> SQCSGIDKRDFIQGVSGGTWVDVVLDRKGCVTISATGKPTIDVRMVKMEASNLASVRTYCLEASTSEISSVNGCPSTTEAHNDKRKDSTYLCERSYPDRGWGNGCGLFGRGSLDTCVKFACSKKMAGHAISRENIVITAAVSVHGHSGAESDDRSQRKSRKELAELTITFKSSIVEADLGDYGKVQFECLMDFGIDLDDVYTADMSGKWWLVKRDWYHDIALPWTAPSADFWHDMDRLVEFSTPHATKQSVYTLGDQEGAMSTALGDAAVIEYMSSGSKVVFRTGFLKCRVKMENLRLKGSTYMQCSKEFSILKRPTATPYGTVIMQVKYAQTDVPCRVPVGVHERPGGEQVGRIITAHPIILQQNDALVIEVEPPFGDSVIEIGLGTTKIVEQWHRDGSSIGAAFTSTMKGVERMALLGEHAWDFGSVGGFFNSMGKAIHSVFGGLFRAVFGGMSW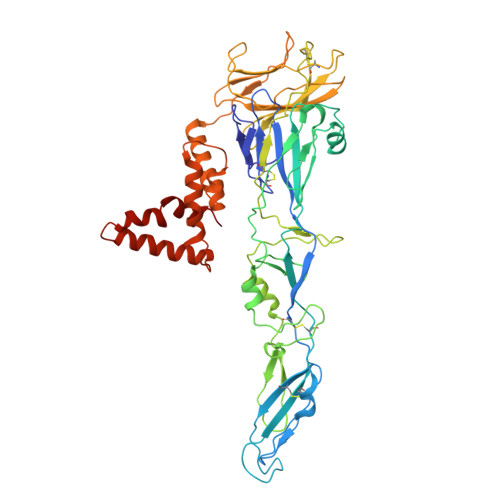ISKVLIGAILMWLGVSAREKTLAMSLITVGAILLYLSTMTNAVS> SADLALGKQTFEANCAACHAGGNNSVIPD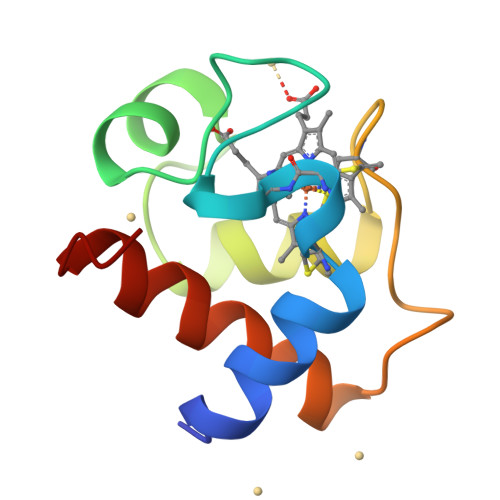HTLRKAAMEQFLQGGFNLEAITYQVENGKGAMPAWSGTLDDDEIAAVAAYVYDQASGDKW4-IODOPYRAZOLE | C3 H3 I N2 | 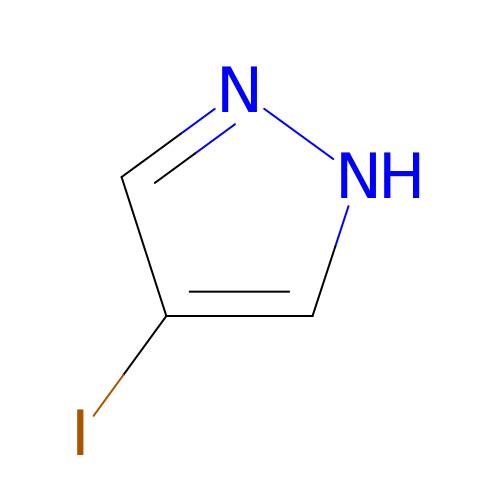LLNQWPTUJJYTTE-UHFFFAOYSA-N>MEKQCSKFIVSGHVQGVGFCYHTSHQGLKLGLTGYAKNLNNGDVEVVACGTPERLEELYLWLQEGPKTA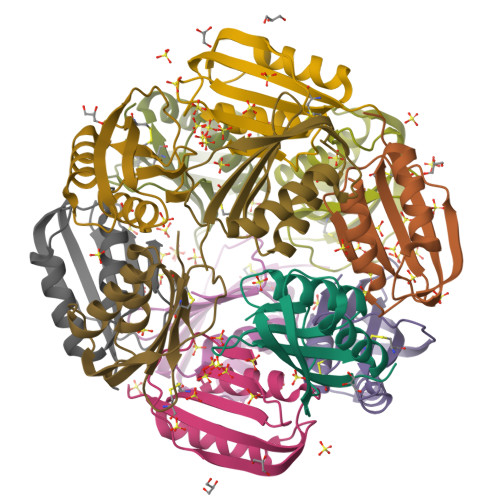SVRQVRRLSSELEHDYQGFEIL[12x]>KESA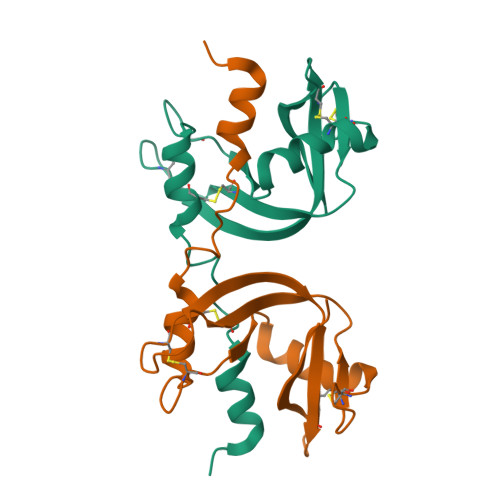AAKFERQHMDSGNSPSSSSTYCNQMMRRRNMTQGRCKPVNTFVHEPLVDVQNVCFQEKVTCKNGQGNCYKSNSSMHITDCRLTNGSRYPNCAYRTSQKERHIIVACEGSPYVPVHFDASVEDST[2x]>PTPVEVSQLTYNADTIGNWVPPTELKQTYTQDITGLKPNSKFIIVPYMDRVSSEVLQKCTITCNEVDAVGSISYFDTSAIKCDGY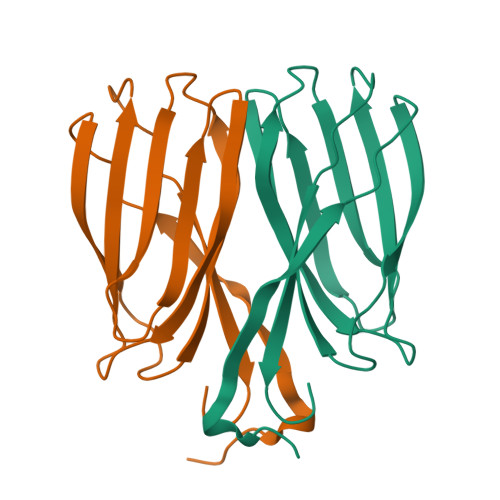ISFQANSIGEATFTLVTDYQGAVDPKPYQYRIIRAIVGNN[8x]> GSGSGTPAPDAINDALRSADSQEARDACQKKGWIVIHPSNELVVEKH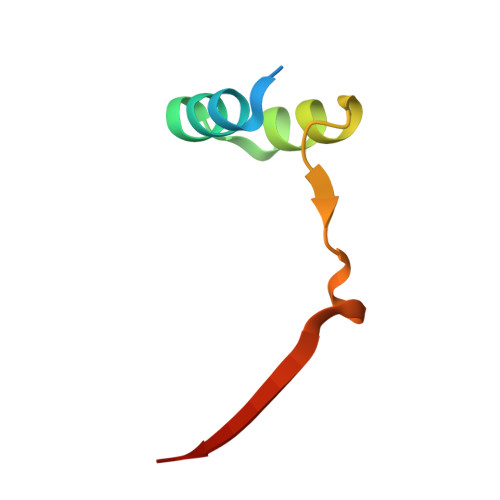ISR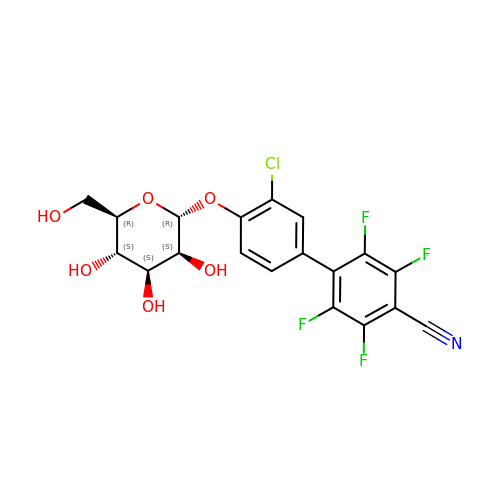4-[3-chloranyl-4-[(2~{R},3~{S},4~{S},5~{S},6~{R})-6-(hydroxymethyl)-3,4,5-tris(oxidanyl)oxan-2-yl]oxy-phenyl]-2,3,5,6-tetrakis(fluoranyl)benzenecarbonitrile | C19 H14 Cl F4 N O6 | TVTALLJBZDAPSI-LCWWKBHCSA-N> GSMSSERVLSYAPAFKSFLDTSFFQELSRLKLDVLKLDSTCQPLTVNLDLHNIPKSADQVPLFLTNRSFEKHNNKRT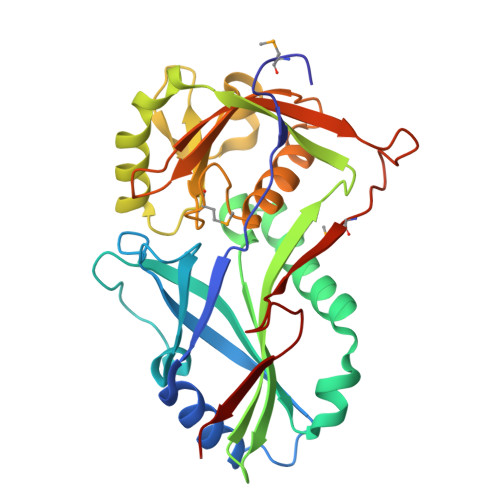NEVPLQGSIFNFNVLDEFKNLDKQLFLHQRALECWEDGIKDINKCVSFVIISFADLKKYRFYYWLGVPCFQRPSSTVLHVRPEPSLKGLFSKCQKWFDVNYSKWVCILDADDEIVNYDKCIIRKTKVLAIRDTSTMENVPSALTKNFLSVLQYDVPDLIDFKLLIIRQNEGSFALNATFASIDPQSSSSNPDMKVSGWERNVQGKLAPRVVDLS> VAETPTYPWRDAETGERLVCAQCPPGTFVQRPCRRDSPTTCGPCPPRHYTQFWNYLERCRYCNVLCGEREEEARACHATHNRACRCRTGFFAHAGFCLEHASCPPGAGVIAPGTPSQNTQCQPCPPGTFSASSSSSEQCQPHRNCTALGLALNVPGS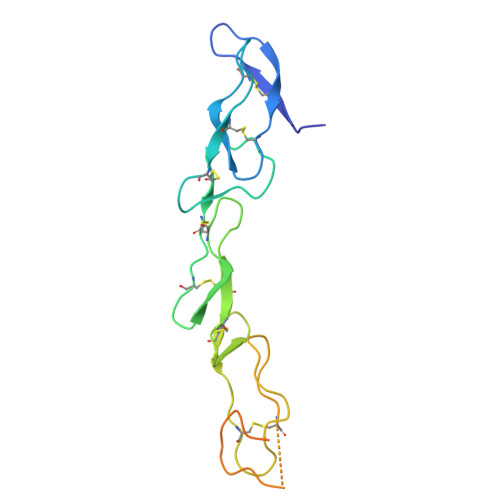SSHDTLCTSTGHHHHHH> GSTGSSKSETTSHTYQHQALVDQLHELIANTDLNKLSYLNLDAFQKRDILAAHYIAKSAIRT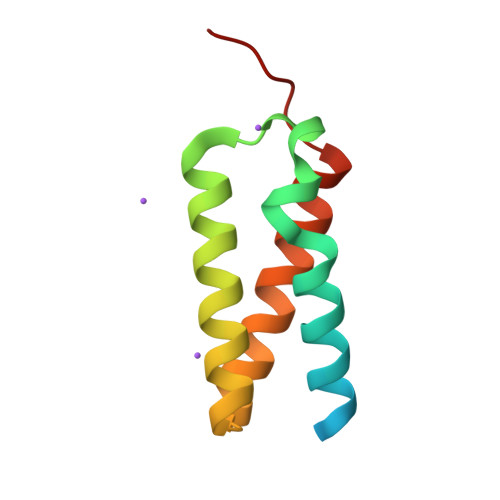KNLDQMTKAKQRLESIYNSISNPLHSQNN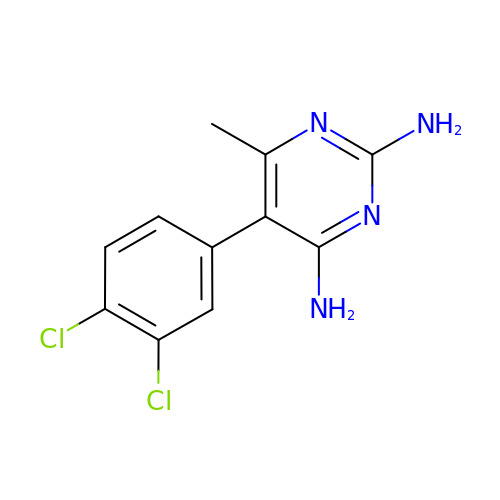5-(3,4-DICHLOROPHENYL)-6-METHYLPYRIMIDINE-2,4-DIAMINE | C11 H10 Cl2 N4 | VQJHOPSWBGJHQS-UHFFFAOYSA-N3-HYDROXY-3-METHYL-GLUTARIC ACID | C6 H10 O5 | 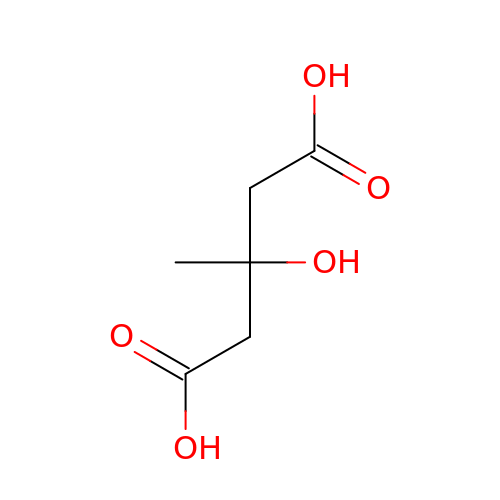NPOAOTPXWNWTSH-UHFFFAOYSA-N>ALGSVTDRHAAEYNMRHKNRGMALIFNHEHFEVPTLKSRAGTNVDCENLTRVLKQLDFEVTVYKDCRYKDILRTIEYAASQNHSDSDCILVAILSHGEMGYIYAKDTQYKLDNIWSFFTANHCPSLAGKPKLFFIQACQGDRLDGGVTMQRSQTETD[2x];>[2x]GDSSMSYKIPVHADFLIAYSTVPGFYSWRNTTRGSWFMQSLCAELAANGKRLDILTLLTFVCQRVAVDFESCTPDTP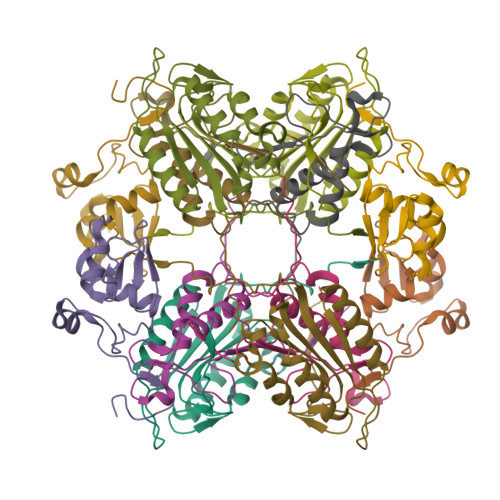EMHQQKQIPCITTMLTRILRFSDKQLAPAGRV;>[2x]NNINKTRMNDLNREETRLKTFTDWPLDWLDKRQLAQTGMYFTHAGDKVKCFFCGVEIGSWEQEDQPVPEHQRWSPNCPLLRRRTTNNVPINAEALDRILPPISYDICGANDSTLE> MRRWHRSLNPALFGERGSGHYFSTTRARLQLQAQDRIICGTHGAGIVAHQTAVNSSDNPMLSSVTTAAPAADLSRTKPHEGTGTSERDPYIRTLHNQRSAAPESSVSQSHTVNAPTVDECEMLAERWGTMNYWHNDTFPRLVVFLKKLLVPDVSPLSPTAESLLSMFEKVVIPKLTSDEEDRRKLVSLWSETTLQAEAAVTKFLFQRGSFESMLHRIITDALEKMSTLALGGQEGNLALEALKRQTLFKRNDYIQKRLIDVVSNSAYLGYGDSVWQVFFAAVEANEENLLSDRATTDAIRAAWEGVM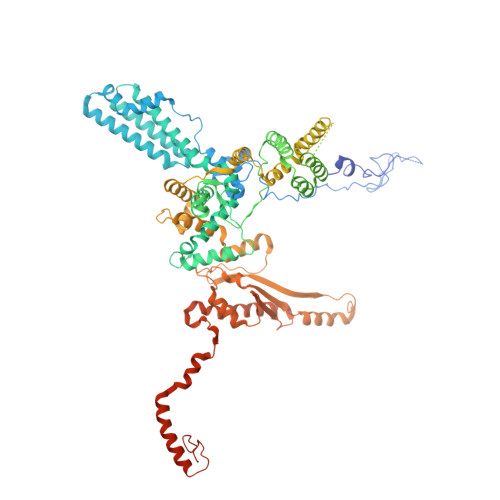REDVVRLPDVTGVVALYLTLVCIRESGRLVPEELKELSSGLEDGVRPGVRKLQQYPLIFLHPTVKRRFVVKAVAEILHNSSSNAFSNMLRENGLHDTAREVALCEAMNRNKELAEGDVGDAVGRFVSKGEVKTLLSSLVSGTDAVVRDAVAGIFGIGTTITIDWDAVMQNVDWSNNWQRLATALLSNSAVLSAIVKLVKNAIGAKGMSKHLFTDEYADQLQLILDAREERAASRKQRIENIAQELSSFERVDLSCDLLRKLGVDMTELDTAAAATRNMNVVQRPCIEDGLLSLVLEAVTKRHPNWVKAGVIQTTLKDPFDALRWMMHIFIRLSYVPHAGAATIARLSRRRIGPIGLEPHQFNVPAELGFVEQYDNLQYKRYDWQGWYQRMLDVHNRNVSLRCRICDLQRLDGNGVQFVDMQTERRLRILAQHRVGMGVLKLDADKYEDQADNVTFGTTKLSELLADARKAQLGEEYWPSVELKVRKPSGQSKAHYSLIDNERIEKRSGELYEKYRDAKKRSLFVTPMETWLEVKGMQVRKSVDNADEDGYTLDALQDMMDGDDGDKV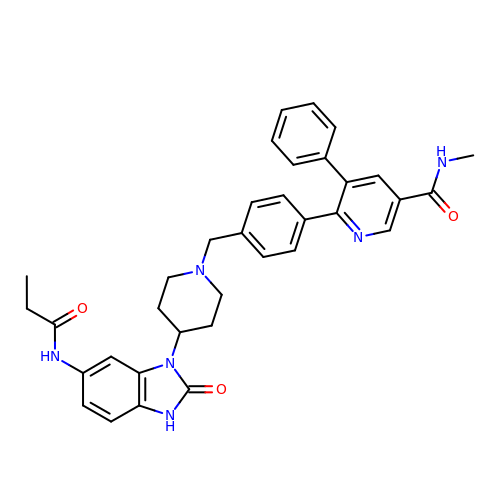~{N}-methyl-6-[4-[[4-[2-oxidanylidene-6-(propanoylamino)-3~{H}-benzimidazol-1-yl]piperidin-1-yl]methyl]phenyl]-5-phenyl-pyridine-3-carboxamide | C35 H36 N6 O3 | DHCFQGXSUHCKEE-UHFFFAOYSA-N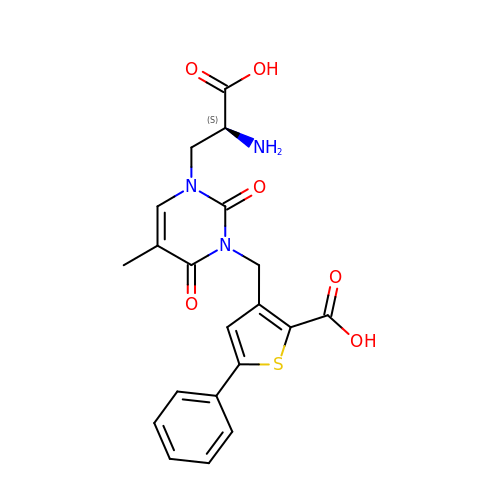3-({3-[(2S)-2-amino-2-carboxyethyl]-5-methyl-2,6-dioxo-3,6-dihydropyrimidin-1(2H)-yl}methyl)-5-phenylthiophene-2-carboxylic acid | C20 H19 N3 O6 S | LCZDCKMQSBGXAH-AWEZNQCLSA-N>G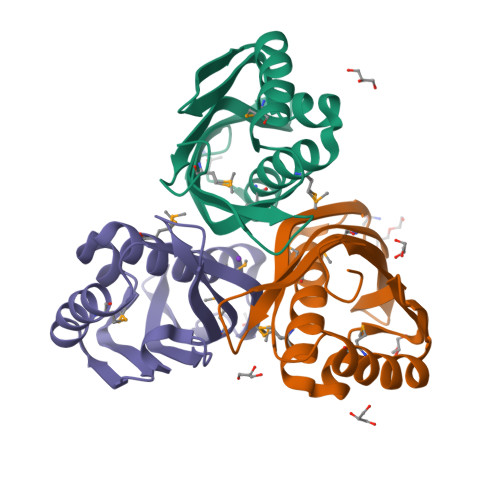MELTALDKLEIMELAARFEMSLDKEDVENYLATFASDGALQGFWGIAKGKEELRQGFYAMLDTFARGKRHCSSNAIIQGNYDEATMESYLTVVNREDLNRAGSAFVKDQVRKINGKWYLILRQIEVDPSLPLLQQSQQAGANA[3x]> MFPKSFMFGASLSGFQFEMGNPNDIKELDTQTDWFVWVRDLENLLNGIVSGDLPENGAWYWRNYEKIHQLAVDFGMDTLRIGIEWSRIFPTSTKEIPFGEGMLEKLDEIANKEAVEHYRKMMEDMKAKGLKVFVNLN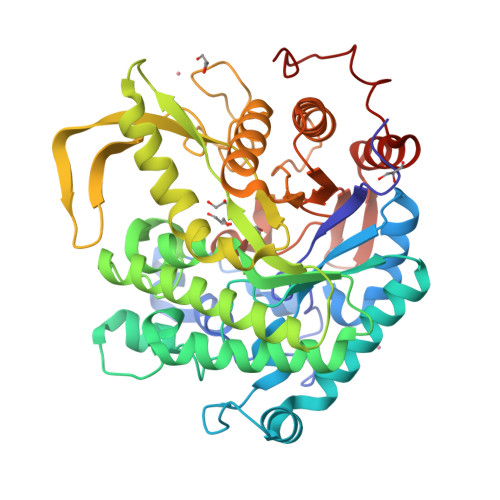HFTLPLWIHDPFAVRKGKPTDKLGWVSDDTPKEFAKYAEYIAWKFSDIVDYWSSMNEPHVVAQLGYFQIMAGFPPNYFNPEWYIKSLKNQALAHNLAYDAIKKHTDKPVGVIYSFTWFDTLKPNDEEIFENAMWLANWNYMDQVKDKIDYIGVNYYTRSVIDKLPTPVNFKDFELNWYTVRGYGYACPEGGFALSGRPASEFGWEIYPEGLYYLLKAIYERYNKPLIVTENGIADEKDKYRSQVIISHLYAVEKAMNEGVDVRGYLHWSIIDNYEWAKGYSKRFGLAYTDLEKKTYIPRPSMYVFREIARTRSIDQFKGYDPYNLMKF> MSLILDDIILSLTNANERTPPQALKTTLSLLYEKSKQYGLSSPQLQALVRLLCETSIIDTVTKVYIVENCFLPDGYLTKELLLEIINHLGTPTVFSRYRIQTPPVLQSALCKWLVHVYFLFPVHSEREHNISSSIWLHLWQFSFLQKWITPLVIWQATTPVDVKPWKLSIIKRCAMHPGYRDAPGSAT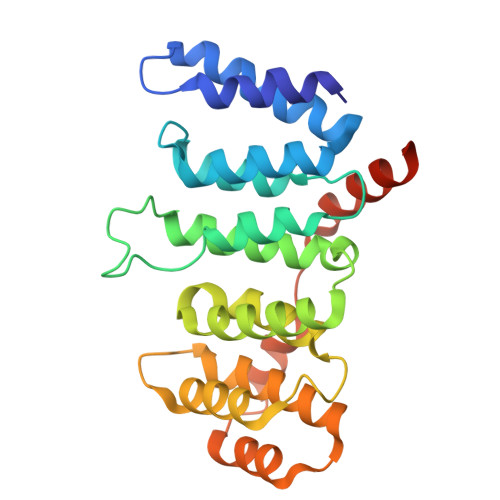LILQRFQCLVGASSQITESIITINCNRKTLKSHRNLKLDAHFLSILKRILSRAHPANENLYFQ>ESSRSAMMYIQELRSGLRDMHLLSCLESLRVSLNNNPVSWVQTFGAEGLASLLDILKRLHDEKEETSGNYDSRNQHEIIRCLKAFMNNKFGIKTMLETEEGILLLVRAMDPAVPNMMIDAAKLLSALCILPQPEDMNERVLEAMTERAEMDEVERFQPLLDGLKSGTSIALKVGCLQLINALITPAEELDFRVHIRSELMRLGLHQVLQELREIENEDMKVQLCVFDEQGDEDFFDLKGRLDDIRMEMDDFGEVFQIILNTVKDSKAEPHFLSILQHLLLVRNDYEARPQYYKLIEECVSQIVLHKNGTDPDFKCRHLQIDIERLVD[4x];>KKVYKPEVQLRRPNWSKFVAEDLSQDCFWTKVKEDRFENNELFAKLTLAFSAQTKTSKAKKDQEGGEEKKSVQKKKVKELKVLDSKTAQNLSIFLGSFRMPYQEIKNVILEVNEAVLTESMIQNLIKQMPEPEQLKMLSELKEEYDDLAESEQFGVVMGTVPRLRPRLNAILFKLQFSEQVENIKPEIVSVTAACEELRKSENFSSLLELTLLVGNYMNAGSRNAGAFGFNISFLCKLRDTKSADQKMTLLHFLAELCENDHPEVLKFPDELAHVEKASRVSAENLQKSLDQMKKQIADVERDVQNFPAATDEKDKFVEKMTSFVKDAQEQYNKLRMMHSNMETLYKELGDYFVFDPKKLSVEEFFMDLHNFRNMFLQAVKENQKRRETEEKM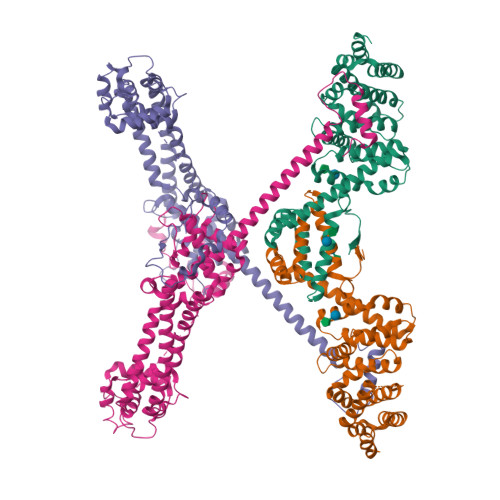RRAKLAKEKAEKERLEKQQKREQLIDMNAEGDETGVMDSLLEALQSGAAFRRKRGPRQVNRKAG[4x]>[6x]MAYTVTN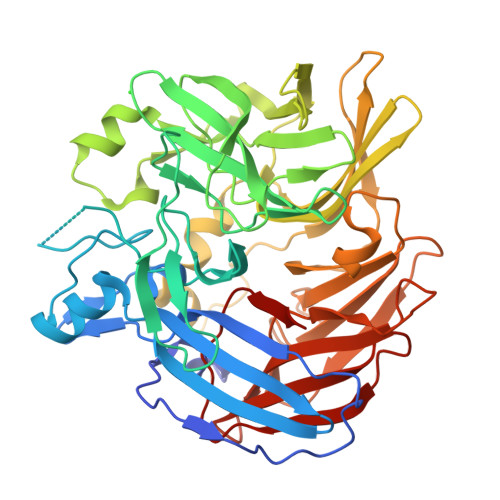KFQLGFSTLSEELDLESLQVKGTIPKWLSGTLIRNGPAKFEVGKEKFQHWFDGLAMLHKFSFKEGKVSYANKFLESKAYQSARDTDKISYREFATDPCRSIFKRVSSMFSTKFTDNANVNVTKIAERFVAMTETPLPVEFDINTLKTVGVFAYDDKIESGLTTAHPHYDFVKNELVNYATKISRSSNYNVYKIADKTNHRNLIGSIPVEEPAYMHSFAMTENYVVLVEYPFVVKPLDLLLSGKPFIENFSWKPENGTRFIIVNRQNGNLVGTYKSDAFFAFHHVNAFEKQEEIFVDIIAYQDSSIVNALYLDILRGQKTDTIPTSHIRRYRIPLSGGQVEYEMLSSEAVELPRINYKQYNTKDYRFVYGISTYSASDFANQLVKIDILRKSSKIWSEKDCYPGEPVFVGAPDATKEDEGLILSAVLDATNAKSFLLILDATTFEEVARAEVPHHIPFGFHGNYFE>[2x]MNVSLQPPPQQLIVQNKTIDLPAVYQLNGGEEANPHAVKVLKELLSGKQSSKKGMLISIGEKGDKSVRKYSRQIPDHKEGYYLSVNEKEIVLAGNDERGTYYALQTFAQLLKDGKLPEVEIKDYPSVRYRGVVEGFYGTPWSHQARLSQLKFYGKNKMNTYIYGPKDDPYHSAPNWRLPYPDKEAAQLQELVAVANENEVDFVWAIHPGQDIKWNKEDRDLLLAKFEKMYQLGVRSFAVFFDDISGEGTNPQKQAELLNYIDEKFAQVKPDINQLVMCPTEYNKSWSNPNGNYLTTLGDKLNPSIQIMWTGDRVISDIT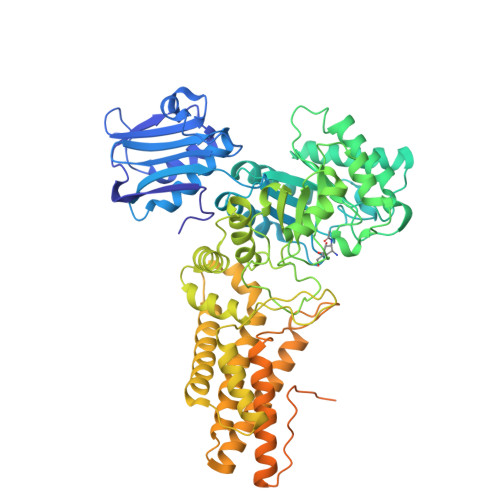RDGISWINERIKRPAYIWWNFPVSDYVRDHLLLGPVYGNDTTIAKEMSGFVTNPMEHAESSKIAIYSVASYAWNPAKYDTWQTWKDAIRTILPSAAEELECFAMHNSDLGPNGHGYRREESMDIQPAAERFLKAFKEGKNYDKADFETLQYTFERMKESADILLMNTENKPLIVEITPWVHQFKLTAEMGEEVLKMVEGRNESYFLRKYNHVKALQQQMFYIDQTSNQNPYQPGVKTATRVIKPLIDRTFATVVKFFNQKFNAHLDATTDYMPHKMISNVEQIKNLPLQVKANRVLISPANEVVKWAAGNSVEIELDAIYPGENIQINFGKDAPCTWGRLEISTDGKEWKTVDLKQKESRLSAGLQKAPVKFVRFTNVSDEEQQVYLRQFVLTIEKK>GNSDDARTSIEQRSNAVSQVLLGIFSYVRWPKEPAVLQLCVVGPTEYADGLLRGMV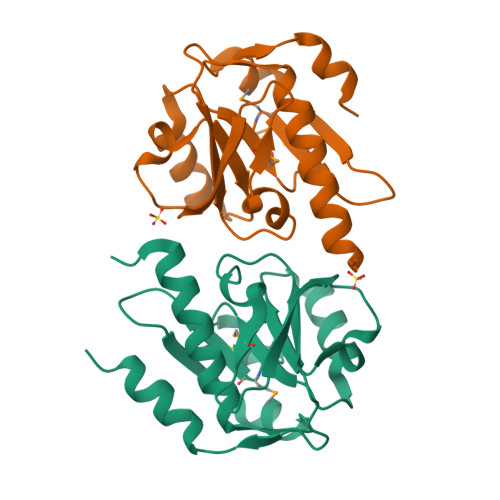QANGRRVHAERRAVDNPDLGTLCNVIYLGVVDERERQQVFRSLAGHPVLSISERGTECSVGSMFCLNVGGPRITFEANLDSIARSGVRVHPSVLKLARRQATP[2x]> MQARARAFRLKSYADGDLLRELRQFDGAKNASELGPRAFVRDSHRLDAAVEKASKLTDPTFHISQYQLPHPYSFGGGPPNPERPLTAPLISAINKVSQRTRDPVGYRKRAKESIDLGDFTTHDPDTLHPRFLEYVHERTRSVDGPTDDAMRAAQTVFARLWRRKGCKVKARSLSDAQPDNLLAIIKKGSPGEYRSLGAEDRRDPRLIATMSSSLLRYASAGVQVARGRPPPGWVDTTTQVTLTFGKREPKAAKIVDGVRQAPVPRFIFNLSPV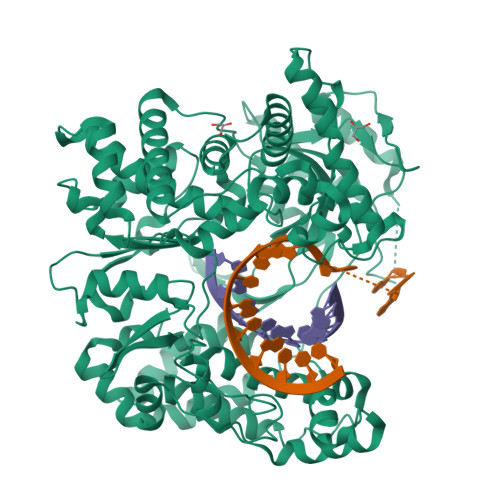NYALASFLHYDISHFLMDNDPTHGPGFGPGRGRARKFMDLVERAFDGRFSTPDGARLIMSDITKWDANMCEALIKYSIDLLEDAVDKSALSPEGLATRGLMYRVARRQLLEKLVEHPAGYFVKLYGCMPSGSFYTSLVNTTGNNLLVIGHAIARAVEETSLTHHGAAELLADAVDGTLISYGDNQLFSEHLFSVLGLAYDPEKHAEFLARFGMKLKVDETEVTVKLGRVRFCSRSLVRTPHGLLITRSHNSLFAKLAGRPRHDPVVDKLYVRAMMVDHMGTDPIVYAILNEIDRSLNVSLEAAGLTDAAKKVLEDTAQSMFGNREQDALLAVYRALSETVIDRRALLSLHTPRDGDHDPGRLHTSVSTGMHLFTGELTPAAQWAYECTVEKWCQYLHDTDQEGVMFDGSSSHHHHHH> GMTTPSHLSDRYELGEILGFGGMSEVHLARDLREHRDVAVKVLRADLARDPSFYLRFRREAQNAAALNHPAIVAVYDTGEAETPAGPLPYIVMEYVDGVTLRDIVHTEGPMTPKRAIEVIADACQALNFSHQNGIIHRDVKPANIMISATNAVKVMDFGIARAIADSGNSVTQTAAV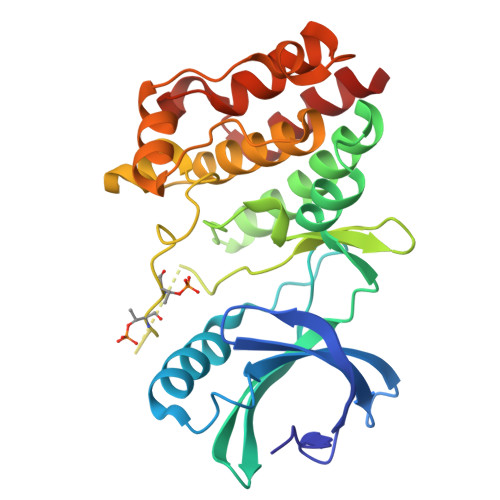IGTAQYLSPEQARGDSVDARSDVYSLGCVLYEVLTGEPPFTGDSPVSVAYQHVREDPIPPSARHEGLSADLDAVVLKALAKNPENRYQTAAEMRADLVRVHNG> MSRSKRDNNFYSVEIGDSTFTVLKR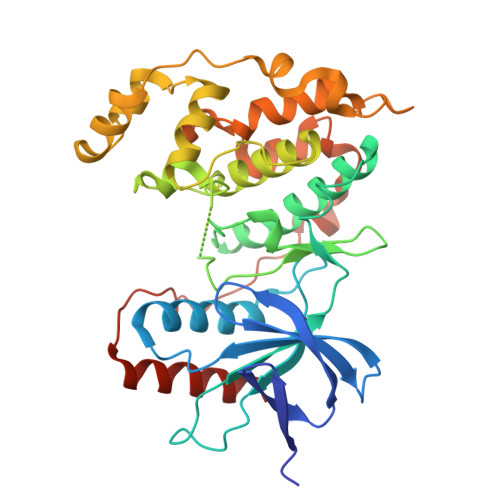YQNLKPIGSGAQGIVCAAYDAILERNVAIKKLSRPFQNQTHAKRAYRELVLMKVVNHKNIIGLLNVFTPQKSLEEFQDVYIVMELMDANLSQVIQMELDHERMSYLLYQMLVGIKHLHSAGIIHRDLKPSNIVVKSDATLKILDFGLARTAGTSFMMTPYVVTRYYRAPEVILGMGYKENVDIWSVGVIMGEMIKGGVLFPGTDHIDQWNKVIEQLGTPSPEFMKKLQPTVRTYVENRPKYAGYSFEKLFPDVLFPADSEHNKLKASQARDLLSKMLVIDASKRISVDEALQHPYINVWYDPSEAEAPPPKIPDKQLDEREHTIEEWKELIYKEVMDLEHHHHHH> AHYNTEILKSIDNEWRKTQCMPREVAIDVGKEFGVATNTFFKPPCVSVYRCGGCCNSEGLQCMNTSTSYLSKTLFEITV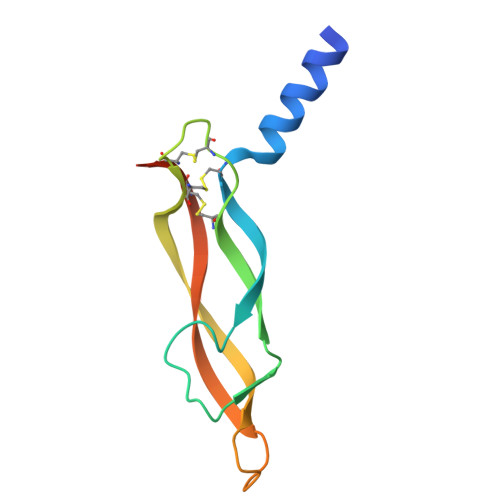PLSQGPKPVTISFANHTSCRCMSKLHHHHHH>[2x]GPLGSPEFMARTLQGEWMKVEQKGGQVPAPRSSHGIAVIGDKLYCFGGEDPPYESIDNDLYVFDFNTHTWSIAPANGDVPKTRVLGTRMVAVGTKLYVFGGRNKQLEFEDFYSYDTVKEEWKFLTKLDEKGGPEARTFHSMTSDENHVYVFGGVSKGGLNATPFRFRTIEAYNIAEGKWAQLPDPGEDFEKRGMAGFLVVQGKLWVFYGFATANDPKIPTLYGSQD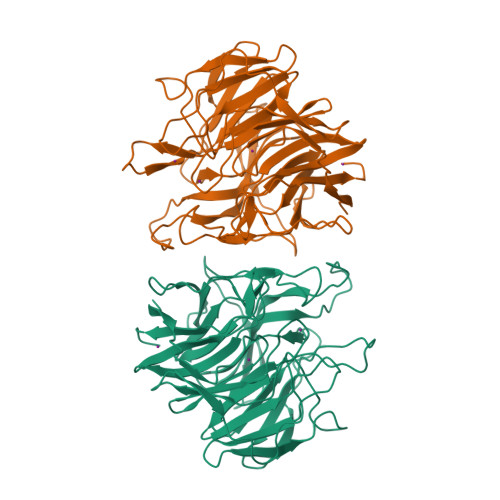YESNRVHCYDPATQKWTEVETTGFEKPSRRSCFAHAAVGKYIIIFGGEIERDPEAHQGPGTLSREGFALDTETLVWERYEGGPIKPSNRGWVASTTTTINGKKGLLVHGGKLMTNERTDEMYFFAVNSST> GFSVDGNTLYDANGQPFVMRGINHGHAWYKDTASTAIPAIAEQGANTIRIVLSDGGQWEKDDIDTIREVIELAEQNKMVAVVEVHDATGRDSRSDLNRAVDYWIEMKDALIGKEDTVIINIANEWYGSWDGSAWADGYIDVIPKLRDAGLTHTLM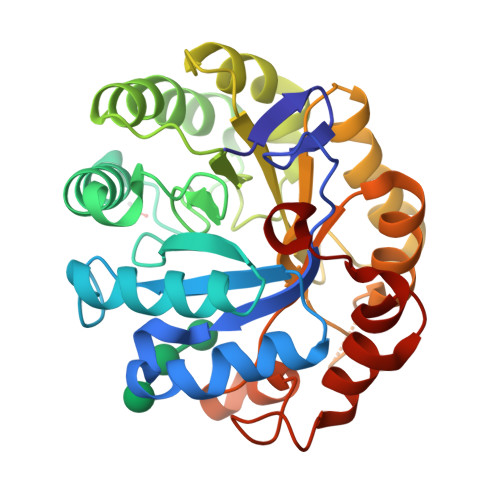VDAAGWGQYPQSIHDYGQDVFNADPLKNTMFSIHMYEYAGGDANTVRSNIDRVIDQDLALVIGEFGHRHTDVDEDTILSYSEETGTGWLAWSWKGNSTSWDYLDLSEDWAGQHLTDWGNRIVHGADGLQETSKPSTVFT> MRVPFSWLKAYVPELESPEVLEERLAGLGFETDRIERVFPIPRGVVFARVLEAHPIPGTRLKRLVLDAGRTVEVVSGAENARKGIGVALALPGTELPGLGQKVGERVIQGVRSFGMALSPRELGVGEYGGGLLEFPEDALPPGTPLSEAWPEEVVLDLEVTPNRPDALGLLGLARDLHALGYALVEPEAALKAEALPLPFALKVEDPEGAPHFTLGYAFGLRVAPSPLWMQRALFAAGMRPINNVVDVTNYVMLERAQPMHAFDLRFVGEGIAVRRAREGERLKTLDGVERTLHPEDLVIAGWRGEESFPLGLAGVMGGAESEVREDTEAIALEVACFDPVSIRKTARRHGLRTEASHRFERGVDPLGQVPAQRRALSLLQALAGARVAEALLEAGSPKPPEAIPFRPEYANRLLGTSYPEAEQIAILKRLGCRVEGEGPTYRVTPPSHRLDLRLEEDLVEEVARIQGYETIPLALPAFFPAPDNRGVEAPYRKEQRLREVLSGLGFQEVYTYSFMDPEDARRFRLDPPRLLLLNPLAPEKAALRTHLFPGLVRVLKENLDLDRPERALLFEVGRVFREREETHLAGLLFGEGVGLPWAKERLSGYFLLKGYLEALFARLGLAFRVEAQAFPFLHPGVSGRVLVEGEEVGFLGALHPEIAQELELPPVHLFELRLPLPDKPLAFQDPSRHPAAFRDLAVVVPAPTPYGEVEALVREAAGPYLESLALFDLYQGPPLP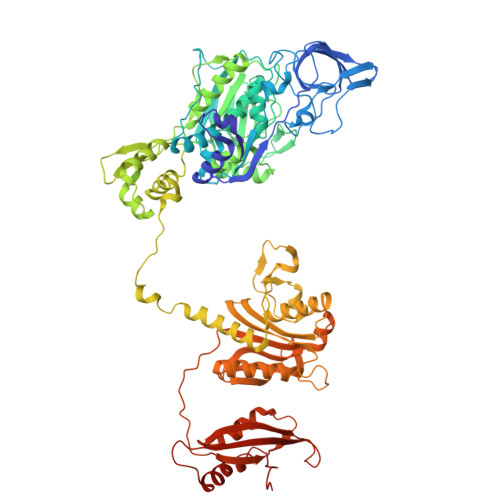EGHKSLAFHLRFRHPKRTLRDEEVEEAVSRVAEALRARGFGLRGLDTP>[2x]KTVNLSACEVAVLDLYEQSNIRIPSDI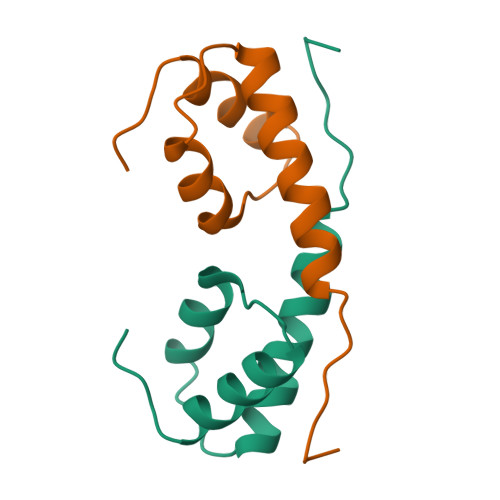IEDLVNQRLQSEQEVLNYIETQRTYWKLENQKKLYRGSLK5'-({[(2R)-3-amino-2-{[2-({N-[(2R)-2-hydroxy-3,3-dimethyl-4-(phosphonooxy)butanoyl]-beta-alanyl}amino)ethyl]sulfanyl}propyl]sulfonyl}amino)-5'-deoxyadenosine 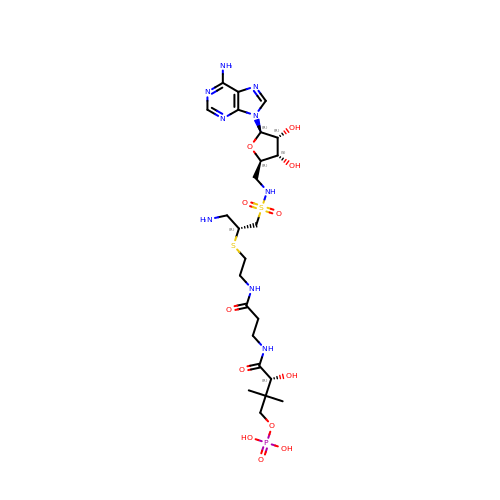| C24 H42 N9 O12 P S2 | AKPDLNPLPXRYTO-XGVFZYDCSA-N> MVDTHKLADDVLQLLDNRIEDNYRVCVILVGSPGSGKSTIAEELCQIINEKYHTFLSEHPNVIEVNDRLKPMVNLVDSLKTLQPNKVAEMIENQGLFKDHVE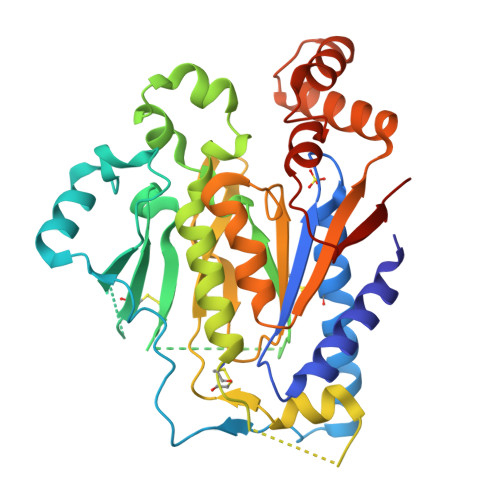DVNFQPVKYSALTSNNEECTAVVARGGTANAIRIAAVDNPVNVNKLAQDSINIAQIVPMDGFHLSRRCLDLFKDPQTAHKRRGSPSTFDSNNFLQLCKILAKTSLCKVSSHHKFYSTSSVFEKLSKTFSQTIPDIFVPGFNHALKDPTPDQYCISKFTRIVILEGLYLLYDQENWKKIYKTLADTGALLVYKIDIDYEATEERVAKRHLQSGLVTTIAEGREKFRSNDLLNGRDIDNHLIKVDNIVHIRNDHHHHHH> MDLVDRAQAGEAEAFGRLYDQYSDTVYRYIYYRVGGKATAEDLTSETFLRALRRISTFTWQGRDFGAWLVTIARNLVAD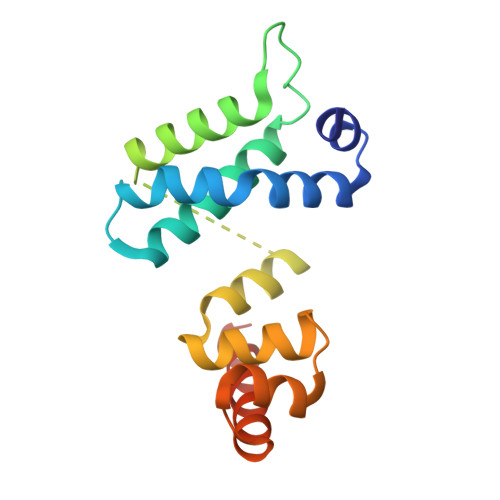HFKSMESLSNAALLDAVRRLNPQQQECVTLRFLQGLSVAETARVMGKNEGAIKTLQYRAVRTLARLLPDDAR> GFPTELKPGTNQFLTTDDGVSAPILPNFHPTPCIHIPGEVRNLLELCQVETILEVNNVPTNATSLMERLRFPVSAQAGKGELCAVFRADPGRNGPWQSTLLGQLCGYYTQWSGSLEVTFMFTGSFMATGKMLIAYTPPGGPLPKDRATAMLGTHVIWDFGLQSSVTLVIPWISNTHYRAHARDGVFDYYTTGLVSIWYQTNYVVPIGAPNT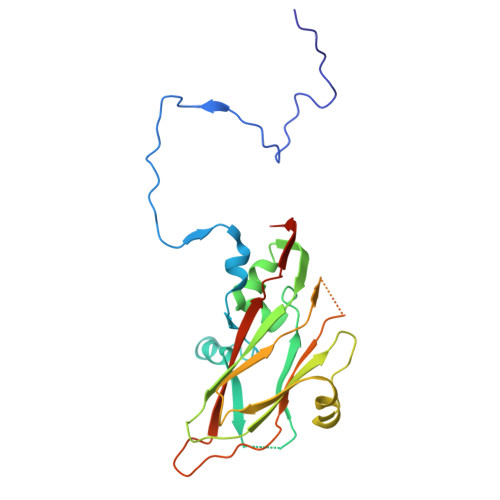AYIIALAAAQKNFTMKLCKDASDILQTG> EEYVGLSANQCAVPAKDRVDCGYPHVTPKECNNRGCCFDSRIPGVPWCFKPLQEAESTLEK

The three human TFFs (TFF1, TFF2, and TFF3)1 are ubiquitous in mucosal environments. The trefoil domain is comprised of three loops (foils) formed by three disulfide bonds. TFF1 and TFF3 are disulfide-linked homo-dimers with each monomer possessing a single trefoil domain, while TFF2 is a single-chain protein with two trefoil domains. Using a combination of ELISA, isothermal titration calorimetry (ITC) and tryptophan quenching assays, we demonstrate that the cognate ligand for all TFFs is the GlcNAc-α-1,4-Gal disaccharide.

Following mTFF3 surface lysine methylation, a crystal of the mTFF3–GlcNAc-α-1,4-Gal complex was obtained and the structure determined to a resolution of 1.55 Å. The disaccharide is accommodated within a hydrophobic cleft of TFF3 with ligand binding driven by sterical fitting and hydrogen bonds to the peptide backbone. Only two side chains, Asp20 and Trp47, make direct contacts with the disaccharide: Asp20 makes a bidentate hydrogen-bonding interaction between O-4 and O-6 of the non-reducing α-GlcNAc, while C-H–π interactions are made between the indole ring of Trp47 and the reducing-end Gal. Trp47 undergoes considerable motion between liganded and unliganded forms. Our structure of TFF3 in complex with GlcNAc-α-1,4-Gal revealed how these simple proteins recognise their disaccharide ligand using just two residue side chains, and how this approach to binding the disaccharide mimics that of the CBM32 domains, which share no sequence or structural similarities with the TFFs. The larger GlcNAc-α-1,4-Gal disaccharide, which is the terminating structure unique to some mucin-like O-glycans, bound to mTFF1, TFF2 and mTFF3 with a Kd of 49 ± 4 µM, 44 ± 8 µM and 65 ± 5 µM, respectively. Using our ELISA, the dTFF1bio-N14A mutant was found to have reduced affinity for pMucinred while the dTFF3bio-D20A mutant had barely any detectable affinity for pMucinred. The dTFF1bio-W41A and dTFF3bio-W47A mutants were also completely inactive by ELISA.>ELKVSLEERDLWTRFKELTNEMIVTKNGRRMFPVLKVSMSGLDPNAMYTVLLDFVAADNHRWKYVNGEWVPGGKPEPQAPSCVYIHPD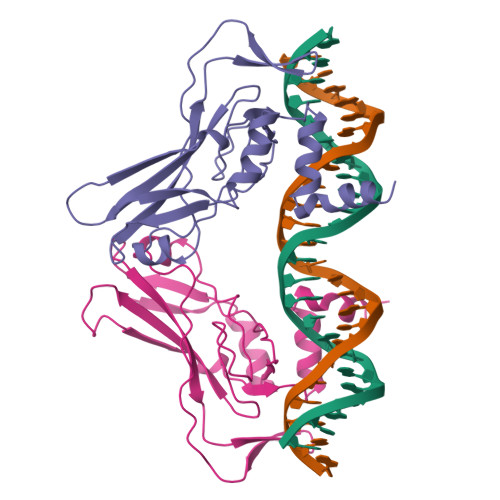SPNFGAHWMKDPVSFSKVKLTNKMNGGGQIMLNSLHKYEPRIHIVRVGGTQRMITSHSFPETQFIAVTAYQNEEITALKIKHNPFAKAFLDAKERN[2x]> FCLTLQNPLRKACISIVEWKPFETIILLTIFANCVALAVYLPMPEDDNNSLNLGLEKLEYFFLTVFSIEAAMKIIAYGFLFHQDAYLRSGWNVLDFIIVFLGVFTAILEQVNVIQSNTAPMSSKGAGLDVKALRAFRVLRPLRLVSGVPSLQVVLNSIFKAMLPLFHIALLVLFMVIIYAIIGLELFKGKMHKTCYYIGTDIVATVENEKPSPCARTGSGRPCTINGSECRGGWPGPNHGITHFDNFGFSMLTVYQCITMEGWTDVLYWVNDAIGNEWPWIYFVTLILLGSFFILNLVLGVLSGEFTKEREKAKSRGTFQKLREKQQLEEDLRGYMSWITQGEVMDVEDLREGKLSLEEGGSDTESLYEIEGLNKIIQFIRHWRQWNRVFRWKCHDLVKSRVFYWLVILIVALNTLSIASEHHNQPLWLTHLQDIANRVLLSLFTIEMLLKMYGLGLRQYFMSIFNRFDCFVVCSGILELLLVESGAMTPLGISVLRCIRLLRLFKITKYWTSLSNLVASLLNSIRSIASLLLLLFLFIIIFALLGMQLFGGRYDFEDTEVRRSNFDNFPQALISVFQVLTGEDWNSVMYNGIMAYGGPSYPGVLVCIYFIILFVCGNYILLNVFLAIAVDNLAEAESLTSAQKAKAEERKRRKMSRGLPDKT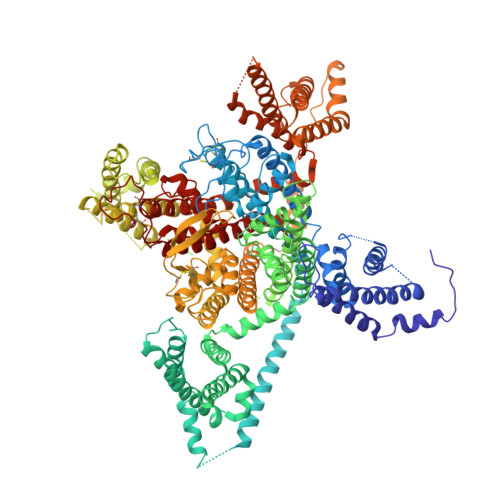EEEKSVMAKKLEQKPKGEGIPTTAKLKVDEFESNVNEVKDPYPSADFPGDDEEDEPEIPVSPRPRPLAELQLKEKAVPIPEASSFFIFSPTNKVRVLCHRIVNATWFTNFILLFILLSSAALAAEDPIRAESVRNQILGYFDIAFTSVFTVEIVLKMTTYGAFLHKGSFCRNYFNILDLLVVAVSLISMGLESSTISVVKILRVLRVLRPLRAINRAKGLKHVVQCVFVAIRTIGNIVLVTTLLQFMFACIGVQLFKGKFFSCNDLSKMTEEECRGYYYVYKDGDPTQMELRPRQWIHNDFHFDNVLSAMMSLFTVSTFEGWPQLLYRAIDSNEEDMGPVYNNRVEMAIFFIIYIILIAFFMMNIFVGFVIVTFQEQGETEYKNCELDKNQRQCVQYALKARPLRCYIPKNPYQYQVWYVVTSSYFEYLMFALIMLNTICLGMQHYHQSEEMNHISDILNVAFTIIFTLEMILKLLAFKARGYFGDPWNVFDFLIVIGSIIDVILSEIDTFLASSGGLYCLGGGCGNVDPDESARISSAFFRLFRVMRLIKLLSRAEGVRTLLWTFIKSFQALPYVALLIVMLFFIYAVIGMQMFGKIALVDGTQINRNNNFQTFPQAVLLLFRCATGEAWQEILLACSYGKLCDPESDYAPGEEYTCGTNFAYYYFISFYMLCAFLIINLFVAVIMDNFDYLT> LLIEPARIEEEELTLTILRQTGGLGISIAGGKGSTPYKGDDEGI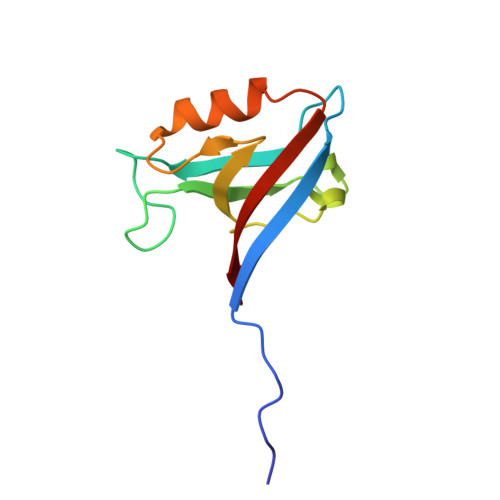FISRVSEEGPAARAGVRVGDKLLEVNGVALQGAEHHEAVEALRGAGTAVQMRVWRERM> MPYSVGFREADAATSFLRAARSGNLDKALDHLRNGVDINTCNQNGLNGLHLASKEGHVKMVVELLHKEIILETTTKKGNTALHIAALAGQDEVVRELVNYGANVNAQSQKGFTPLYMAAQENHLEVVKFLLENGANQNVATEDGFTPLAVALQQGHENVVAHLINYGTKGKVRLPALHIAARNDDTRTAAVLLQNDPNPDVLSKTGFTPLHIAAHYENLNVAQLLLNRGASVNFTPQNGITPLHIASRRGNVIMVRLLLDRGAQIETKTKDELTPLHCAARNGHVRISEILLDHGAPIQAKTKNGLSPIHMAAQGDHLDCVRLLLQYDAEIDDITLDHLTPLHVAAHCGHHRVAKVLLDKGAKPNSRALNGFTPLHIACKKNHVRVMELLLKTGASIDAVTESGLTPLHVASFMGHLPIVKNLLQRGASPNVSNVKVETPLHMAARAGHTEVAKYLLQNKAKVNAKAKDDQTPLHCAARIGHTNMVKLLLENNANPNLATTAGH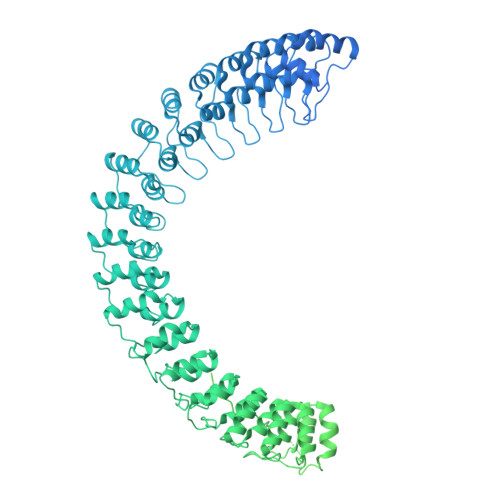TPLHIAAREGHVETVLALLEKEASQACMTKKGFTPLHVAAKYGKVRVAELLLERDAHPNAAGKNGLTPLHVAVHHNNLDIVKLLLPRGGSPHSPAWNGYTPLHIAAKQNQVEVARSLLQYGGSANAESVQGVTPLHLAAQEGHAEMVALLLSKQANGNLGNKSGLTPLHLVAQEGHVPVADVLIKHGVMVDATTRMGYTPLHVASHYGNIKLVKFLLQHQADVNAKTKLGYSPLHQAAQQGHTDIVTLLLKNGASPNEVSSDGTTPLAIAKRLGYISVTDVLKVVTDETSFVLVSDKHRMSFPETVDEILDVSEDEGEELISFKAERRDSRDVDEEKELLDFVPKLDQVVESPAIPRIPCAMPETVVIRSEEQEQASKEYDEDSLIPSSPATETSDNISPVASPVHTGFLVSFMVDARGGSMRGSRHNGLRVVIPPRTCAAPTRITCRLVKPQKLSTPPPLAEEEGLASRIIALGPTGAQFLSPVIVEIPHFASHGRGDRELVVLRSENGSVWKEHRSRYGESYLDQILNGMDEELGSLEELEKKRVCRIITTDFPLYFVIMSRLCQDYDTIGPEGGSLKSKLVPLVQATFPENAVTKRVKLALQAQPVPDELVTKLLGNQATFSPIVTVEPRRRKFHRPIGLRIPLPPSWTDNPRDSGEGDTTSLRLLCSVIGGTDQAQWEDITGTTKLVYANECANFTTNVSARFWLSDCPRTAEAVNFATLLYKELTAVPYMAKFVIFAKMNDPREGRLRCYCMTDDKVDKTLEQHENFVEVARSRDIEVLEGMSLFAELSGNLVPVKKAAQQRSFHFQSFRENRLAMPVKVRDSSREPGGSLSFLRKAMKYEDTQHILCHLNITMPPCAKGSGAEDRRRTPTPLALRYSILSESTPGSLSGTEQAEMKMAVISEHLGLSWAELARELQFSVEDINRIRVENPNSLLEQSVALLNLWVIREGQNANMENLYTALQSIDRGEIVNMLEGSGRQSRNLKPDRRHTDRDYSLSPSQMNGYSSLQDELLSPASLGCALSSPLRADQYWNEVAVLDAIPLAATEHDTMLEMSDMQVWSAGLTPSLVTAEDSSLECSKAEDSDATGHEWKLEGALSEEPRGPELGSLELVEDDTVDSDATNGLIDLLEQEEGQRSEEKLPGSKRQDDATGAGQDSENEVSLVSGHQRGQARITHSPTVSQVTERSQDRLQDWDADGSIVSYLQDAAQGSWQEEVTQGPHSFQGTSTMTEGLEPGGSQEYEKVLVSVSEHTWTEQPEAESSQADRDRRQQGQEEQVQEAKNTFTQVVQGNEFQNIPGEQVTEEQFTDEQGNIVTKKIIRKVVRQIDLSSADAAQEHEEVTVEGPLEDPSELEVDIDYFMKHSKDHTSTPNP> MTNLAPANSEKIRVDIWSDIACPWCYIGKRRFESALGQFPQRDQV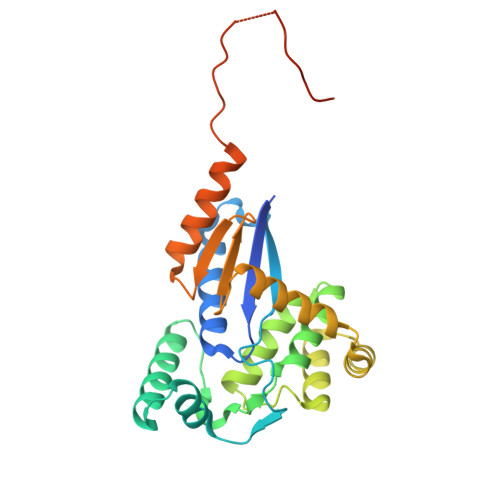EVVWHSFELDPSARPLNPIAMRDGLAMKYSISPAQAQGSLDHMTQTAAQEGLEYHFDRVKLANTFLAHQLIHYAAEQGQGDAMKERLLRAYMSEGQNVNDLDTLQKLAAEVGLDAGAARAALEAGTYAQAVRYDEAQAQQLGITGVPFFVLGGKYGVSGAQAPETLLGALSQVWAEQHPAPLTMLGQDAPAEGCEDGQCAVPQRPNNLEHHHHHH>MSAQKRITLYMASASPFPHRVRLALEEAHATYEMIHISLVDKQDWYQKKVYPDRAQVPYLIYGGPELHPDEAPS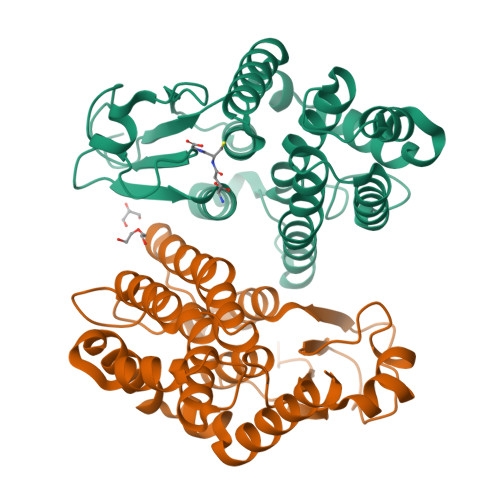PDAAKIPESLVILEFLADLFPAAHLLPSDPVLRARARLFTTAVETELLPAQKAFFLMGGPPDAMLAALDALQARLPPAGGFAAGPQWSIADAAVMPILLRLRMSVTLEVGFFAPGAAPVVRAALESPRFARLQRYIADNVARPSMAATWDEAAVKAEFVGRFEKLRSLKAAQHHHHHH[2x]>MWSHPAVRKSSSKTIRSRSIWDDAHAMLEKAKAEGISTVWDRAAEQTPACKFCELGTTCRNCIMGPCRIANRKDGKMRLGVCGADADVIVARNFGRFIAGGAAGHSDHGRDLIETLEAVAEGKAPGYTIRDVAKLRRIAAELGVADAATRPAHDVAADLVTICYNDFGSRRNALAFLARAPQVRRDLWQRLGMTPRGVDREIAEMMHRTHMGCDNDHTSLLVHAARTALADGWGGSMIGTELSDILFGTPRPRQSTVNLGVLRKDAVNILVHGHNPVVSEMILAATREPAVRQAAQDAGAADINVAGLCCTGNELLMRQGIPMAGNHLMTELAIVTGAADAIVADYQCIMPSLVQIAACYHTRFVTTSPKGRFTGATHVEVHPHNAQERCREIVMLAIDAYTRRDPARVDIPSQPVSIMSGFSNEAILEALGGTPKPLIDAVVAGQIRGFVGIVGCNNPKIRQDSAN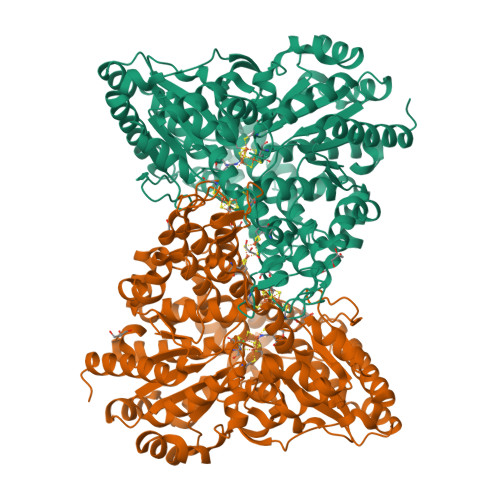VTLTRELIRRDIMVLATGCVTTAAGKAGLLVPEAASKAGEGLAAVCRSLGVPPVLHMGSCVDNSRILQLCALLATTLGVDISDLPVGASSPEWYSEKAAAIAMYAVASGIPTHLGLPPNILGSENVTAMALHGLQDVVGAAFMVEPDPVKAADMLEAHIVARRARLGLTS[2x]[2-(ethylsulfonyl)phenyl][(2S)-4-(6-fluoro-1,3-benzothiazol-2-yl)-2-methylpiperazin-1-yl]methanone | 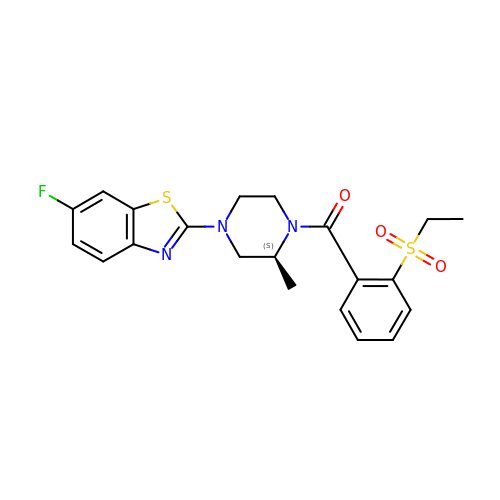C21 H22 F N3 O3 S2 | UKQOLPNYRVPCBM-AWEZNQCLSA-N>IGVCYGMSANNLPAASTVVSMFKSNGIKSMRLYAPNQAALQAVGGTGINVVVGAPNDVLSNLAASPAAAASWVKSNIQAYPKVSFRYVCVGNEVAGGATRNLVPAMKNVHGALVAAGLGHIKVTTSVSQAILGVFSPPSAGSFTGEAAA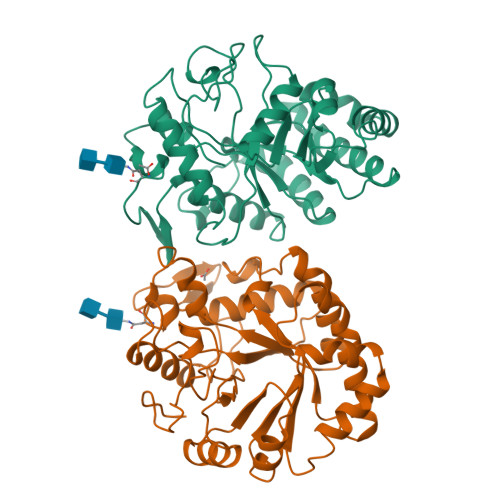FMGPVVQFLARTNAPLMANIYPYLAWAYNPSAMDMGYALFNASGTVVRDGAYGYQNLFDTTVDAFYTAMGKHGGSSVKLVVSESGWPSGGGTAATPANARFYNQHLINHVGRGTPRHPGAIETYIFAMFNENQKDSGVEQNWGLFYPNMQHVYPINF[2x]> QDPIKFTTGSATPASYNQFIDALRERLTGGLIYGIPVLRDPSTVEKPNQYVTVELSYSDTVSIQLGIDLTNAYVVAYRAGSESFFFRNAPASASTYLFTGTQQYSLPFDGNYDDLEKWAHQSRQRISLGLEALRQGIKFLRSGASDDEEIARTLIVIIQMVAEAARFRYVSKLVVISLSNRAAFQPDPSMLSLENTWEPLSRAVQHTVQDTFPQNVTLINVRQERVVVSSLSHPSVSALALMLFVCNPLNATQSPLLIRS;> VVEQSKICSSHYEPTVRIGGRDGLCVDVSDNAYNNGNPIILWKCKDQLEVNQLWTLKSDKTIRSKGKCLTTYGYAPGNYVMIYDCSSAVAEATYWDIWDNGTIINPKSGLVLSAESSSMGGTLTVQKNDYRMRQGWRTGNDTSPFVTSIAGFFKLCMEAHGN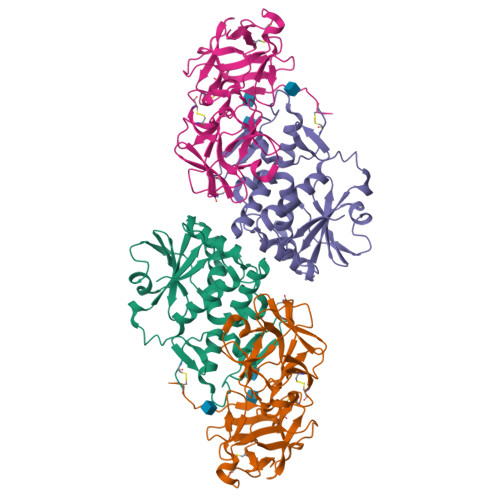SMWLDVCDITKEEQQWAVYPDGSIRPVQNTNNCLTCEEHKQGATIVMMGCSNAWASQRWVFKSDGTIYNLYDDMVMDVKSSDPSLKQIILWPYTGNANQMWATLF>GAMGTRDDEYDYLFKVVLIGDSGVGKSNLLSRFTRNEFNLESKSTIGVEFATRSIQVDGKTIKAQIWDTAGQERYRAITSAYYRGAVGALLVYDIAKHLTYENVERWLKELRDHADSNIVIMLVGNKSDLRHLRAVPTDEARAFAEKNGLSFIETSALDSTNVEAAFQTILTEIYRIVS[3x];>[3x]GAMGSVNIPRKEKDFQGMLEYKKEDEQKLVKNLILELKPRGVAVNLIPGLPAYILFMCVRHADYLNDDQKVRSLLTSTINSIKKVLKKRGDDFETVSFWLSNTCRFLHCLKQYSGEEGFMKHNTSRQNEHCLTNFDLAEYRQVLSDLAIQIY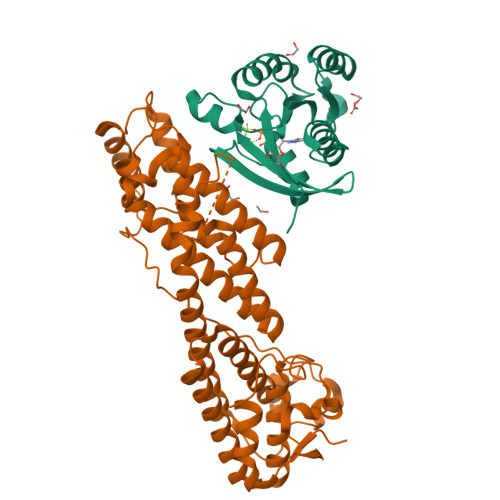QQLVRVLENILQPMIVSGMLEHETIQGVSGVKPTGLRKRTSSIADEGTYTLDSILRQLNSFHSVMCQHGMDPELIKQVVKQMFYIIGAITLNNLLLRKDMCSWSKGMQIRYNVSQLEEWLRDKNLMNSGAKETLEPLIQAAQLLQVKKKTDDDAEAICSMCNALTTAQIVKVLNLYTPVNEFEERVSVSFIRTIQMRLRDRKDSPQLLMDAKHIFPVTFPFNPSSLALETIQIPASLGLGFISRV> MSLNGITKYVEKLTFFNIQSGKQVEFNRDEKVILSNVPFIQQLPELD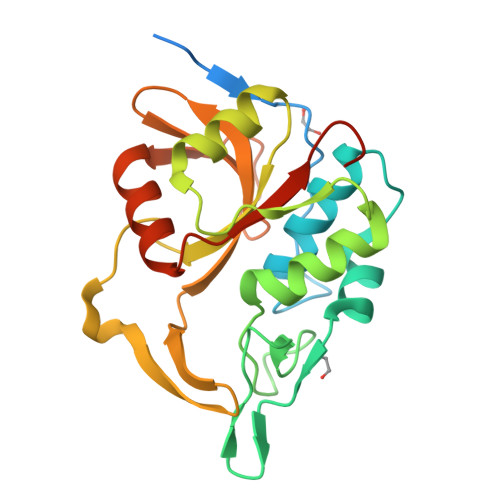RGCEVTSLAMMLQYAGITVDKMKLANEIKKVDFMNDGVRGNPNEGFVGNIYTFSESGYGVYHGPLFQLAKKYLPNKAVDLTGKSIEELYKSVKAGQPVVIITNATFAPLDEDEFTTWETNNGDVSITYNEHCVVLIGYDQESVYIRDPLKDSLDVKVPREKFEQAWVQMGSQAISYVKRSKEGHHHHHH>[8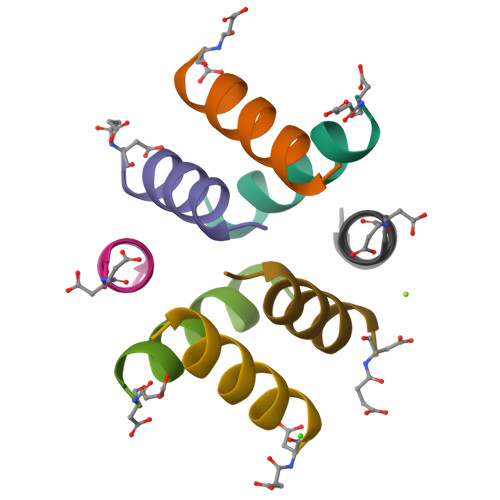x]DELERAIRELAARIKX> PVPR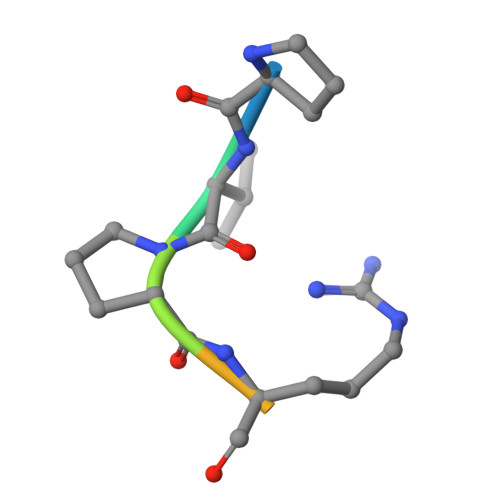AHS>YKEEDSTVSILPTSLPQIHRANMLAQGSPAASKISPLVTKKSKTRWHFGIRSRSYPLDVMGEIYIALKNLGAEWAKPSEEDLWTIKLRWKYDIGNKTNTNEKIPDLMKMVIQLFQIETNNYLVDFKFDGWESSYGDDTTVSNISEDEMSTFSAYPFLHLTTKLIMELAVNS[2x];>SLMVPVEIRWQQGGSKVYVTGSFTKWRKMIGLIPDSDNNGSFHVKLRLLPGTHRFRFIVDNELRVSDFLPTATDQMGNFVNYIEVRQPEKNPTNEKIRSKEADSMRPPTSDRSSIALQIGKDPDDFGDGYTRFHEDLSPRPPLEYTTDIPAVFTDPSVMERYYYTLDRQQSNTDTSWLTPPQLPPQLENVILNKYYATQDQFNENNSGALPIPNHVVLNHLVTSSIKHNTLCVASIVRYKQKYVTQILYTPI[2x];>SQEKVSIEQQLAVESIRKFLNSKTSYDVLPVSYRLIVLDTSLLVKKSLNVLLQNSIVSAPLWDSKTSRFAGLLTTTDFINVIQYYFSNPDK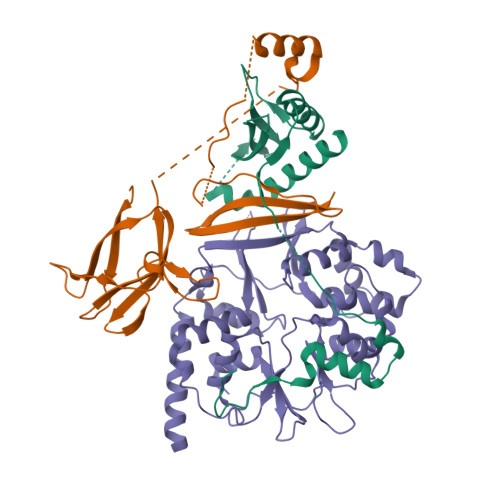FELVDKLQLDGLKDIERALGVDQLDTASIHPSRPLFEACLKMLESRSGRIPLIDQDEETHREIVVSVLTQYRILKFVALNCRETHFLKIPIGDLNIITQDNMKSCQMTTPVIDVIQMLTQGRVSSVPIIDENGYLINVYEAYDVLGLIKGGIYNDLSLSVGEALMRRSDDFEGVYTCTKNDKLSTIMDNIRKARVHRFFVVDDVGRLVGVLTLSDILKYILLGS[2x]2-{[(4-O-alpha-D-glucopyranosyl-beta-D-glucopyranosyl)oxy]methyl}-2-octyldecyl 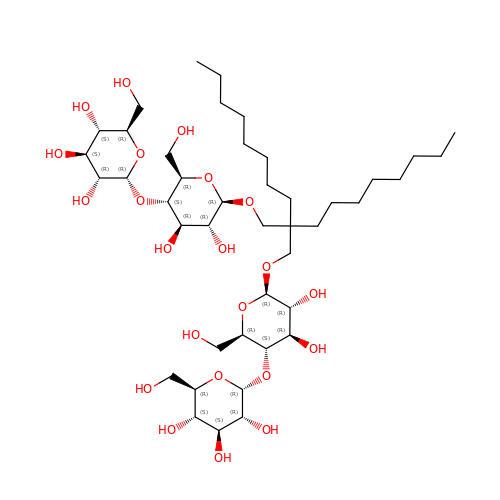4-O-alpha-D-glucopyranosyl-beta-D-glucopyranoside | C43 H80 O22 | GDAZOFIUKHGYGD-VLJUBQHSSA-N>[2x]MGLDSSHVGVRPSPATSQPTTSTGSADLDSILGHMGLPLGNSVLVE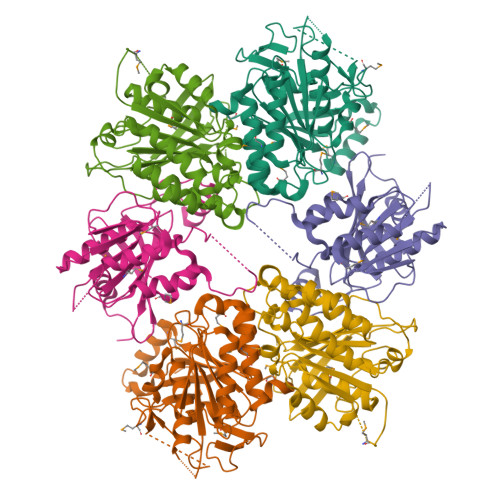EQSTTEFHSILGKLFAAQGIVHNRISDSSADKTRNGDTHVIVLSLNQMFAKELPGIYKGSRKQMKKNLISEEESKVTVQNLNETQRSTPSRYKDLKIAWKYKLADEKRLGSPDRDDIQQNSEYKDYNHQFDITTRLMPAPIASELTFIAPTQPVSTILSQIEQTIKRNDKKLIRIVIPSLLHPAMYPPKMFESSEIIGLMHGVRSLVKKYYERVVLFASISIDIITPPLLVLLRNMFDSVINLEPFNQEMTEFLERVYKSQPGKIQHGLVHILKLPVFTDRGEMRVLKSEWAFKNGRKKFEIEQWGIPVDDAEGS;>[2x]MASSSHNPVILLKRILSLTESSPFILCLDSIAQTSYKLIQEFVHQSKSKGNEYPIVYISFETVNKPSYCTQFIDATQMDFVHLVKQIISYLPAATATQAKKHMVIIDSLNYISTEYITRFLSEIASPHCTMVATYHKDIKDENRTVIPDWNNNYPDKLTLLQFMATTIVDIDVVLTGTLDTEEVSELLNEFRIPRGLNNDIFQLRLVNKRKSGRSLEYDFIVNSNTHEYELLSTTKQEEESSSNGLETPEMLQGLTTFNLGTSNKQKLAK;>MHHHHHHMGSVQRQDLVLFSDQSVLPAHFFQDSNSHNLFFITHQSCTQPLWMINALVETHVLGSPSSLNESSSSMLPSSTRSHAVLASFIHEQNYFTNSLNKLKIPSNNYNVLDFLSDFIVNNIHNKPRDKILSDVLAKFSAAIQNNPTDTIVIIEQPELLLSLVSGLTCSELNNKFITPLLRQCKVLIIVSNSDIFNIDEYDASVHSSNLQNFYKSSFIKSMINLNLNPLKTGFAKDVTGSLHVCRGGAPIATSNTSLHVVENEYLYLNEKESTKLFYR[2x]>APTIPQGQGKVTFNGTVVDAPCSISQKSADQSIDFGQLSKSFLEAGGVSKPMDLDIELVNCDITAFKGGNGAKKGTVKLAFTGPIVNGHSDELDTNGGTGTAIVVQGAGKNVVFDGSEGDANTLKDGENVLHYTAVVKKSSAVGAAVTEGAFSAVANFNLTYQ[13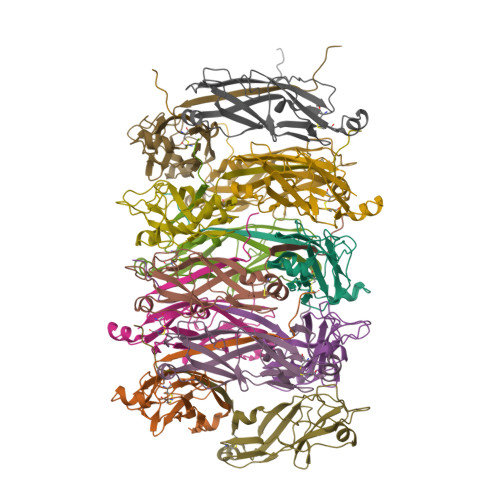x]> MSKIKLTILQVGEENWATKENIPNNMEWLFIKPDQISDFVTTENNYLTSSKLLQKLPRKISALLLTEQTYGPELSSLSSFFEVYEVFYPKDKHATGITEEFLRSKMAQRYDSSSPDQLIRQFYKGLFIGQYGEKLQVSQIQIRNDFEGVVNYQGNNYLELEGQFGENYSFLLNFAYNIPFSSDFYNELFLEHIIEGDIDIRLVISLIVDGSVDDIAKEWYFEKEDLNQLISLESDISGSLAVKLFAKGKGIVKLGPLHRRNGRGGLGTFLLGGERHIDAIGHEFMTYFDPVDFKPPLTVYFSGFRSAEGFEGFWMMKSMKTPFMLICDPRLQGGAFYIGSKEYEQKIVDAIQEKLAFLNFSSDQLILSGLSMGTYGATYHGAKLNPHAIIIGKPIFNLGTVAQRERLERPDGFATSLDIQLLNQGDLTSSSSEKLNNYFWKSIEEGDFSNTTFALAYMKNDDYDAT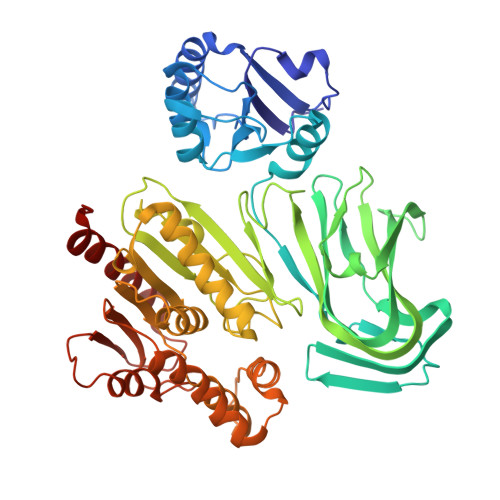AFSDLLQYFRGKKHKILGRGWDGRHGDCSAEVGAWFTSQYRRMLSNDFGRKEE> SARPSSSMADFRKFFAKAKHIVIISGAGVSAESGVPTFRGAGGYWRKWQAQDLATPLAFAHNPSRVWEFYHYRREVMGSKEPNAGHRAIAECETRLGK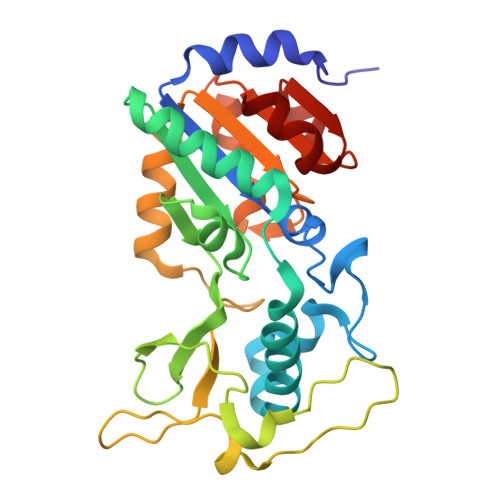QGRRVVVITQNIDELHRKAGTKNLLEIHGSLFKTRCTSCGVVAENYKSPICPALSGKGAPEPGTQDASIPVEKLPRCEEAGCGGLLRPHVVWFGENLDPAILEEVDRELAHCDLCLVVGTSSVVYPAAMFAPQVAARGVPVAEFNTETTPATNRFRFHFQGPCGTTLPEALA>GSMTSKIALFDQTLIASLLQPLSLNQPDFKAYKTKVKLKISEQRNETSGEKELKFEISRSDDFEFLFSETLNNEKYQILARDHDLTVDFDAFPKVIIQHLLCKNTEINIILDAEKNFCSFELFSKTPGSKGKIFSIKLHAVRGDHLISHLLKICSSQAVKLSTFYKSADELASLRQKCGDLEKQ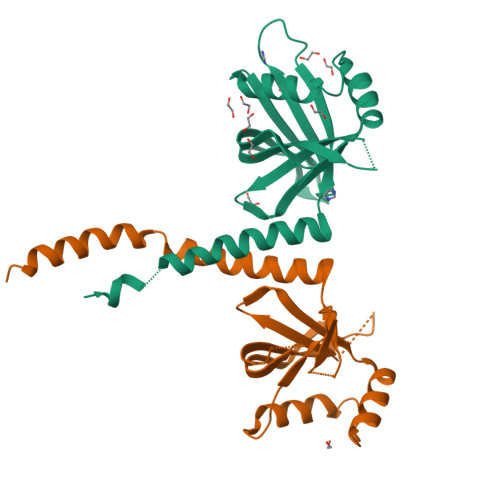VEKLS[2x]>AQADGAKIYAQCAGCHQQNGQGIPGAFPPLAGHVAEILAKEGGREYLILVLLYGLQGQIEVKGMKYNGVMSSFAQLKDEEIAAVLNHIATAWGDAKKVKGFKPFTAEEVKKLRAKKL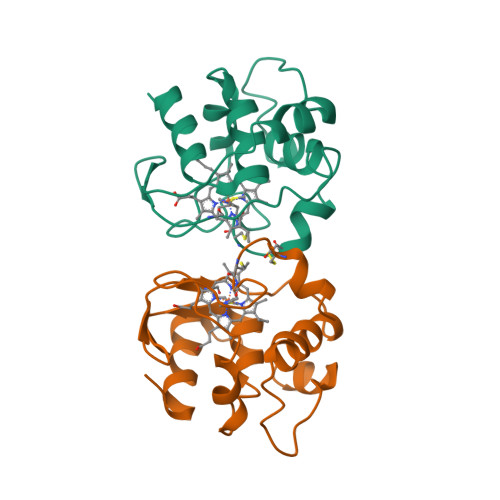TPQQVLAERKKLGLK[2x]Pyruvate dehydrogenase complex (PDHc) is a large multienzyme assembly (Mr = 4–10 million Daltons) consisting of three essential components: pyruvate dehydrogenase (E1p), dihydrolipoyl transacetylase (E2p), and dihydrolipoyl dehydrogenase (E3). These three enzymes perform distinct functions sequentially to catalyze the oxidative decarboxylation of pyruvate with formation of nicotinamide adenine dinucleotide (NADH) and acetyl-coenzyme A. By irreversibly converting the main product of glycolysis to precursors of tricarboxylic acid cycle, PDHc controls the carbon flux in carbohydrate catabolism and act as a gatekeeper to maintain glucose homeostasis. Mammalian E2p and E3BP jointly assemble into a 60-mer icosahedral core scaffold with their C-terminal inner core (IC) domains. Exterior to the core, E1p and E3 are noncovalently anchored to the peripheral subunit binding domains (PSBD) of E2p and E3BP, respectively, forming a flexible outer shell around inner scaffold.

To investigate the overall architecture of native mammal PDHc, we have extracted endogenous PDH complexes from porcine (Sus scrofa) myocardium based on a conventional method of mitochondrial multienzyme isolation. We then collected 11,575 cryo-EM micrographs of purified PDHc and processed the dataset with single-particle analysis (SPA). Averaging images from 2D classification revealed that while the internal densities maintained a regularly ordered configuration, the external densities appeared irregular and diffuse, indicating that peripheral subunits exhibited significantly mobility and were non-identical among complexes. We thereby masked the external densities and conventionally enforced ortho-icosahedral symmetry to determine the IC structure at a resolution of 3.66 Å. Similar to those of Homo sapiens and Bos taurus, the porcine PDHc core presented a tightly stacked dodecahedral scaffold, consisting of 60 repeating IC domains, in which C-terminal region of E2p (residues 418–646) was appropriately fitted, whereas the N-terminal regions, including LD domains, PSBD domain, and their inter-domain linkers, were excluded due to their conformational flexibility. Within this reconstruction, adjacent IC domains are compactly trimerized to form a dodecahedron vertex, which visually resembled a tripetalous, pyramid-like structure with a height of 70 Å and a diameter of 80 Å, reminiscent of homologous structures in the cubic cores of A. vinelandii E2p. Comparable intra-interactions were detected in porcine E2p vertex, wherein each trimer, with a total buried area of 4,272 Å2, incorporated multiple inter-domain interactions at four different regions to maintain structural stability. These twenty vertexes were organized into scaffold assemblies through hydrophobic interactions, with a classical double-handed manner.

>[60x]MWRVCARRAQNAAPRAGFGARWTALREEPGAPCAAPRAGSVPARCSSTTRGYGRSRALCGWSASSWATPQNRILLQLWGSPNRRWYSLPPHQKVPLPSLSPTMQAGTIARWEKKEGDKINEGELIAEVETDKATVGFESLEECYMAKILVAEGTRDVPVGAIICITVEKPEDIEAFKNYTLDSSAAPAPQAAPAPTPAAAAPAPTPSAQAPGSSYPTHMQVVLPALSPTMTMGTVQRWEKKVGEKLSEGDLLAEIETDKATIGFEVQEEGYLAKILIPEGTRDVPLGTPLCIIVEKEADIPAFADYRPTEVTDLKPPAPPPTPSPVTPVPPAPQPVAPTPAATRPATPAGPKGRLFVSPLAKKLASEKGIDLTQIKGTGPDGRIIKKDIDSFVPTKAAPTPAAAVPPPSPGVAPVPTGVFTDIPISNIRRVIAQRLMQSKQTIPHYYLSVDVNMGEVLLVRKELNKMLEGRSKISVNDFIIKASALACLKVPEANSSWLDTVIRQNHVVDISVAVSTPAGLITPIVFNAHIKGLETIANDVVSLATKAREGKLQPHEFQGGTFTISNLGMFGIKNFSAIINPPQACILAVGASEDRLFPADNEKGFDVASMMSVTLSCDHRVVDGAVGAQWLAEFRKYLEKPITMLL>[2x]SMALGPFPAMENQVLVIRIKIPNSGAVDWTVHSGPQLLFRDVLDVIGQVLPEATTTAFEYEDED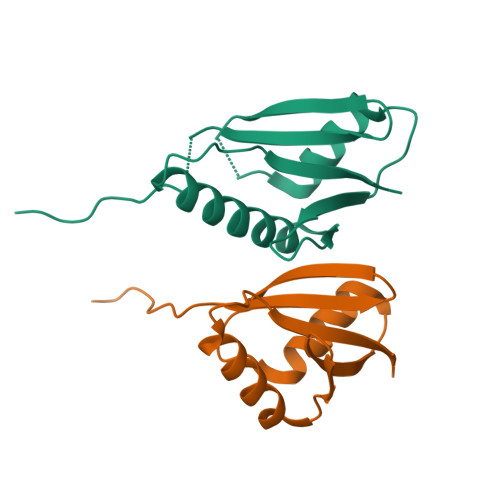GDRITVRSDEEMKAMLSYYYSTVMEQQVNGQLIEPLQIFPRA;>[2x]SMSLQETRKAKSSSPKKQNDVRVKFEHRGEKRILQFPRPVKLEDLRSKAKIAFGQSMDLHYTNNELVIPLTTQDDLDKAVELLDRSIHMKSLKILLVING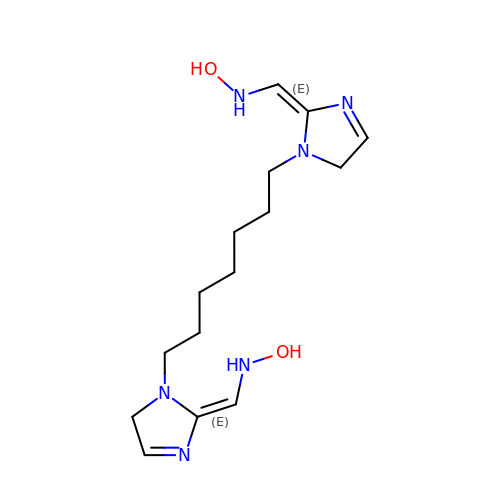(Z,Z)-[heptane-1,7-diylbis(1H-imidazol-1-yl-2-ylidene)]bis(N-hydroxymethanamine) | C15 H26 N6 O2 | XUMCQYQLNOCDFI-QUMQEAAQSA-N>IVGGYNCEENSVPYQVSLNSGYHFCGGSLINEQWVVSAGHCYKSRIQVRLGEHNIEVLEGNEQFINAAKIIRHPQYDRKTLNNDIMLIKLSSRAVINARVSTISLPTAPPATGTKCLISGWGNTASSGADYPDELQCLDAPVLSQAKCEASYPGKITSNMFCVGFLEG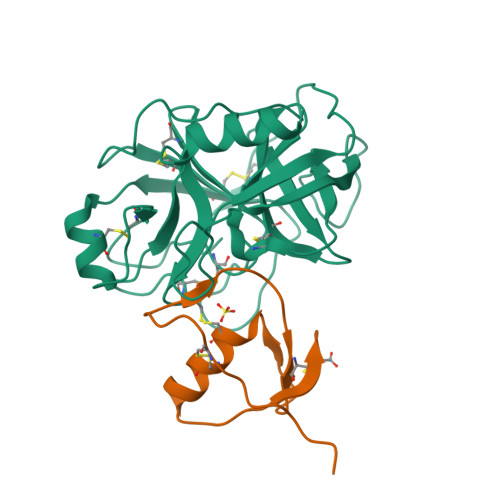GKDSCQGDAGGPVVCNGQLQGVVSWGDGCAQKNKPGVYTKVYNYVKWIKNTIAANS[2x];>[2x]DSLGREAKCYNELNGCTKIYDPVCGTDGNTYPNECVLCFENRKRQTSILIQKSGPC>[2x]MHHHHHHDDDDKRTLPGEGTQVHPRAPL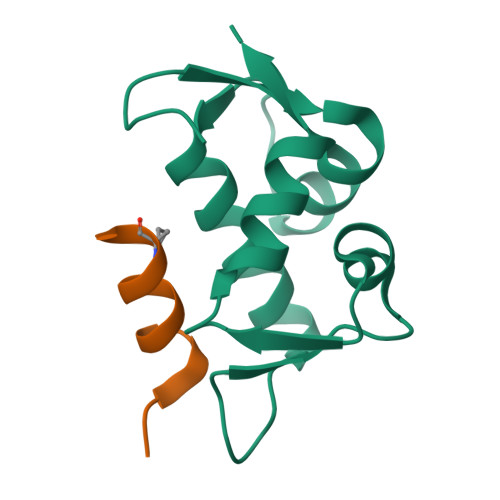LQILKVAGAQEEVFTVKEVMHYLGQYIMMKQLYDKQRQHIVHCHDDPLGELLEVGSFSVKNPSPLYEMLKRNLVIL;>[2x]QSQQTFXNLWRLLLQNX> SKTITLYLDPASLPALNQLMDFTQNNEDKTHPRIFGLSRFKIPDNIITQYQNIHFVELKDNRPTEALFTILDQYPGNIELNIHLNIAHSVQLIRPILAYRFKHLDRVSIQQLNLYDDGSMEYVDLEKE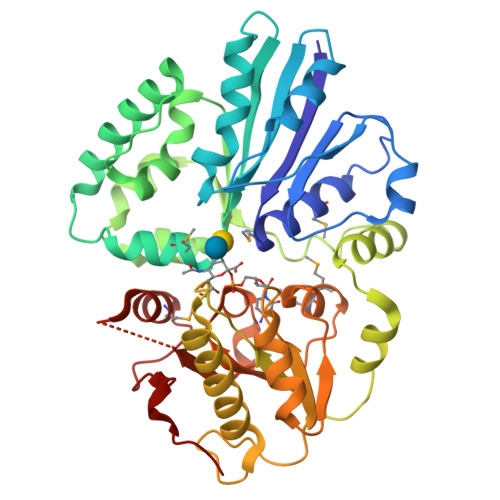ENKDISAEIKQAEKQLSHYLLTGKIKFDNPTIARYVWQSAFPVKYHFLSTDYFEKAEFLQPLKEYLAENYQKMDWTAYQQLTPEQQAFYLTLVGFNDEVKQSLEVQQAKFIFTGTTTWEGNTEVREYYAQQQLNLLNHFTQAEGDLFIGDHYKIYFKGHPRGGEINDYILNNAKNITNIPANISFEVLMMTGLLPDKVGGVASSLYFSLPKEKISHIIFTSNKQVKSKEDALNNPYVKVMRRLGIIDESQVIFWDSLKELG3,3-DIMETHYLBUTAN-1-OL | C6 H14 O | 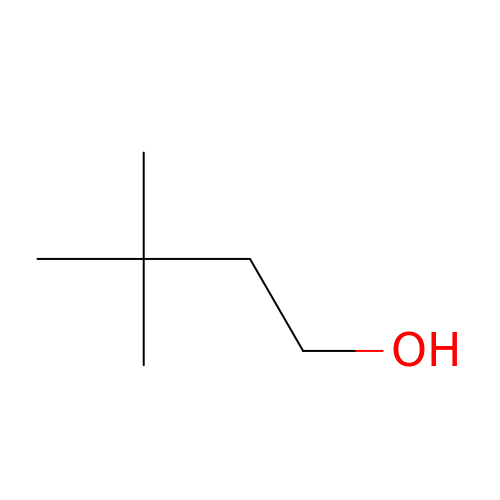DUXCSEISVMREAX-UHFFFAOYSA-N>MQTQILERMESEVRTYSRSFPTVFTEAKGARLHAEDGNQYIDFLAGAGTLNYGHNHPKLKQALADYIASDGIVHGLDMWSAAKRDYLETLEEVILKPRGLDYKVHLPGPTGTNAVE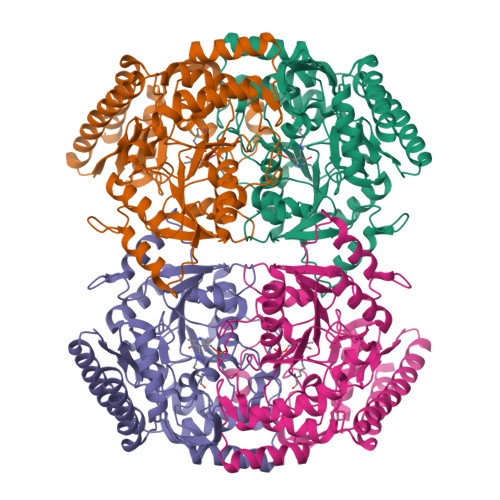AAIRLARNAKGRHNIVTFTNGFHGVTMGALATTGNRKFREATGGIPTQGASFMPFDGYMGEGVDTLSYFEKLLGDNSGGLDVPAAVIIETVQGEGGINPAGIPWLQRLEKICRDHDMLLIVDDIQAGCGRTGKFFSFEHAGITPDIVTNSKSLSGFGLPFAHVLMRPELDIWKPGQYNGTFRGFNLAFVTAAAAMRHFWSDDTFERDVQRKGRVVEDRFQKLASFMTEKGHPASERGRGLMRGLDVGDGDMADKITAQAFKNGLIIETSGHSGQVIKCLCPLTITDEDLVGGLDILEQSVKEVFGQAHHHHHH[8x]> HHHHHHGSGTNVNDKVTASNFKLEKTTFDPNQSGNTFMAANFTVTDKVKSGDYFTAKLPDSLTGNGDVDYSNSNNTMPIADIKSTNGDVVAKATYDILTKTYTFVFTDYVNNKENINGQFSLPLFTDRAKAPKSGTYDANINIADEMFNNKITYN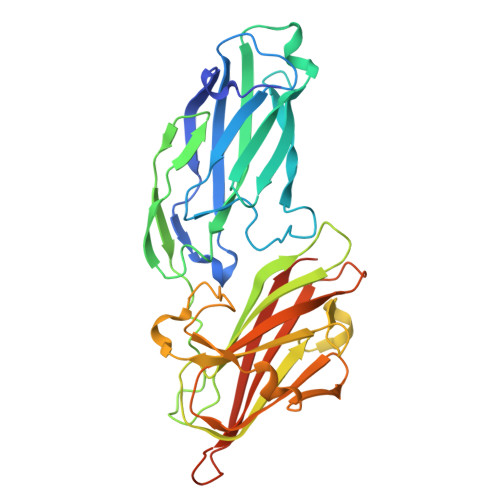YSSPIAGIDKPNGANISSQIIGVDTASGQNTYKQTVFVNPKQRVLGNTWVYIKGYQDKIEESSGKVSATDTKLRIFEVNDTSKLSESYYADPNDSNLKEVTDQFKNRIYYEHPNVASIKFGDITKTYVVLVEGHYDNTGKNLKTQVIQENVDPVTNRDYSIFGWNNENVVRYGGGSADGDSAV> MGSDKIHHHHHHMSRQANRGTESKKMSSELFTLTYGALVTQLCKDYENDEDVNKQLDRMGYNIGVRLIEDFLARSNVGRCHDFRETADVIAKVAFKMYLGITPSITNWSPAGD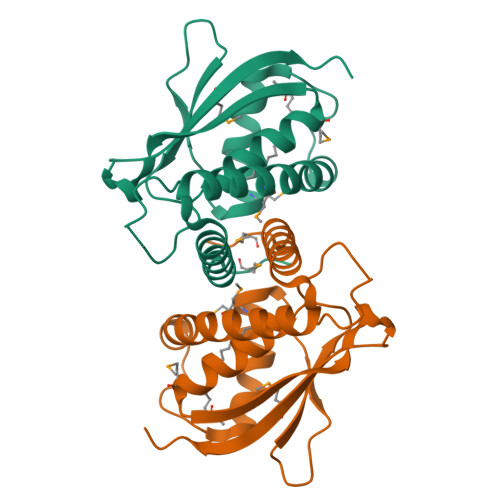EFSLILENNPLVDFVELPDNHSALIYSNLLCGVLRGALEMVQMAVEAKFVQDTLKGDGVTEIRMRFIRRIEDNLPAGEE The histone chaperone FACT plays an important role in facilitating nucleosome assembly and disassembly during transcription. FACT is a heterodimeric complex consisting of Spt16 and SSRP1. Spt16 consists of an NTD followed by an SSRP1 dimerization domain, MD and C-terminal domain. The N-terminal domain of Spt16 resembles an inactive aminopeptidase.

Here, the crystal structure of the N-terminal domain (NTD) of human Spt16 is reported at a resolution of 1.84 Å. Our human Spt16 NTD construct consists of residues 1–510. While the construct contains residues 1–510, electron density for residues 433–510 was not visible. The structure of human Spt16 NTD reveals two lobes: an N-lobe comprising residues 1–175 and a C-lobe comprising residues 176–432. The structure adopts an aminopeptidase-like fold similar to those of the Saccharomyces cerevisiae and Schizosaccharomyces pombe Spt16 NTDs. Despite the presence of a linker between the two lobes, the orientation of the two lobes appears to be rigid across the three Spt16 NTD structures. Isothermal titration calorimetry analyses show that human Spt16 NTD binds histones H3/H4 with low-micromolar affinity, suggesting that Spt16 NTD may contribute to histone binding in the FACT complex. An ITC experiment with human Spt16 NTD against H2A/H2B showed very little change in enthalpy when Spt16 NTD was added to H2A/H2B, suggesting that Spt16 NTD does not bind H2A/H2B or binds with a very weak affinity. Surface-residue conservation and electrostatic analysis reveal a conserved acidic patch that may be involved in histone binding.

> AVTLDKDAYYRRVKRLYSNWRKGEDEYANVDAIVVSVGVDEEIVYAKSTALQTWLFGYELTDTIMVFCDDKIIFMASKKKVEFLKQIANTKGNENANGAPAITLLIREKNESNKSSFDKMIEAIKESKNGKKIGVFSKDKFPGEFMKSWNDCLNKEGFDKIDISAVVAYTIAVKEDGELNLMKKAASITSEVFNKFFKERVMEIVDADEKVRHSKLAESVEKAIEEKKYLAGADPSTVEMCYPPIIQSGGNYNLKFSVVSDKNHMHFGAITCAMGIRFKSYCSNLVRTLMVDPSQEVQENYNFLLQLQEELLKELRHGVKICDVYNAVMDVVKKQKPELLNKITKNLGFGMGIEFREGSLVINSKNQYKLKKGMVFSINLGFSDLTNKEGKKPEEKTYALFIGDTVLVDEDGPATVLTSVKKKVKNVGIFL The condensin protein complex plays a key role in the structural organization of genomes. Based on their homology to ATP binding cassette (ABC) transmembrane transporters and the Rad50 DNA damage repair protein, the two globular ATPase “head” domains situated at the ends of ∼50-nm-long intra-molecular coiled coils of a heterodimer of condensin’s Smc2 and Smc4 subunits are thought to sandwich a pair of ATP molecules between composite catalytic sites, each composed of Walker A (P loop) and Walker B motifs of one head and a so-called ABC signature motif of the opposite head. Each head domain (hd) can be subdivided into a “RecA”-like lobe that contains the ATP-binding pocket and a “helical” lobe that merges into the coiled coils; they connect the heads to a half-doughnut-shaped “hinge” dimerization domain. Smc2hd and Smc4hd are furthermore connected by their binding to opposite ends of the Brn1Cnd2/NCAPH kleisin subunit (Onn et al., 2007).

To gain functional insights into the condensin ATPase cycle, we solved the crystal structures of Smc2hd and the Smc4hd-Brn1C complex of the thermophilic yeast Chaetomium thermophilum (Ct) to 2.6- or 3.0-Å resolution, respectively. As expected, both structures revealed canonical two-lobed SMC ATPase folds that display a high degree of evolutionary surface conservation at their ATP-binding and head dimerization interfaces. Although included in the crystallization construct, crystals of the Ct Smc2hd domain showed no electron density for the N-terminal Brn1 region, which presumably dissociated during crystallization (see below). A comparison of the nucleotide-free Ct Smc2hd and Smc4hd–Brn1C structures of condensin to the adenosine 5′-[γ-thio]triphosphate (ATPγS)-bound Saccharomyces cerevisiae (Sc) Smc1hd-Scc1C and Smc3hd-Scc1N structures of cohesin or to bacterial SMC ATPase head structures revealed differences in the orientations of the helical lobes and attached coiled coils relative to the RecA lobes, which can be explained by flexion movements of ∼25° or ∼15°, respectively. These motions displace strictly conserved glutamine residues in the Smc2 and Smc4 Q loops, which are thought to coordinate the catalytic Mg2+ ion and contribute to nucleotide binding. In contrast, even the wild-type (WT) version of Ct Smc2hd-Brn1N was unable to bind ATP. This finding is readily explained by the Ct Smc2hd structure, where the more pronounced flexion of the Smc2 helical lobe not only repositions the Q loop but also induces a cascade of structural displacement events that alter the P loop of the ATP-binding pocket into a conformation that is incompatible with nucleotide binding. The Smc2 head fails to bind ATP on its own, presumably because of the deformation of the Smc2 P loop observed in two different crystal forms, but readily binds and hydrolyses ATP when in complex with the Smc4 head.

> MRVTELIIDGFKSYAVRTVITGWDESFNAVTGLNGSGKSNILDAICFVLGITNMSTVRAQNLQDLIYKRGQAGVTKASVTIVFDNRDKKRSPIGFEEYATISVTRQIVLGGTTKYLINGHRAQQQTVQNLFQSVQLNINNPNFLIMQGRITKVLNMKPAEILAMIEEAAGTRMFEDRKEKALKTMAKKDLKLQEITELLADEIEPKLEKLRQEKRAFLDFQQTQSGGSGGSLRKKINPKVMNMIDSVEKKEMSLKHMMKTVLKDKHKIEETIATLDEYKRKALQETWEKVNGDFGQIFNELLPGSFAKLEPPEGKDLTDGLEVKVRLGKVWKQSLTELSGGQRSLIALSLIMALLQFKPAPMYILDEVDAALDLSHTQNIGRLIKTRFKGSQFIVVSLKDGMFQNANRIFRVRFSEGTSVVQALTPADLK>[2x]DFEYLQLVLTWPASFCYANHCERIAPNNFTIHGLWPDNVKTRLHNCKPKPTYSYFTGKMLNDLDKHWMQLKFEQDYGRTEQPSWKYQYIKHGSCCQKRYNQ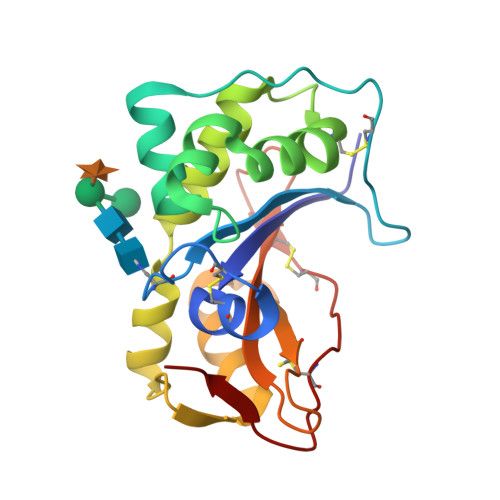NTYFGLALRLKDKFDLLRTLQTHRIIPGSSYTFQDIFDAIKTVSQENPDIKCAEVTKGTPELYEIGICFTPNADSMFRCPQSDTCDKTAKVLFRR>[2x]TTVYYDQDVKTDALQGKKIAVVGYGSQG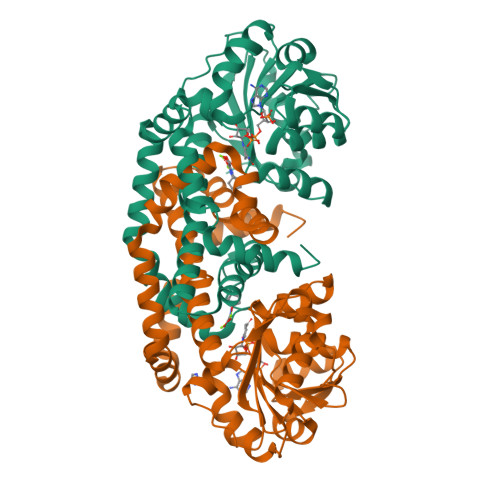HAHAQNLKDNGYDVVIGIRPGRSFDKAKEDGFDVFPVAEAVKQADVIMVLLPDEIQGDVYKNEIEPNLEKHNALAFAHGFNIHFGVIQPPADVDVFLVAPKGPGHLVRRTFVEGSAVPSLFGIQQDASGQARNIALSYAKGIGATRAGVIETTFKEETETDLFGEQAVLCGGVSKLIQSGFETLVEAGYQPELAYFEVLHEMKLIVDLMYEGGMENVRYSISNTAEFGDYVSGPRVITPDVKENMKAVLTDIQNGNFSNRFIEDNKNGFKEFYKLREEQHGHQIEKVGRELREMMPFIKSKSIEKHHHHHH>[2x]MDYKDDDDKWSHPQFEKHHHHHHHHWSHPQFEKQPPPPGPLGDCLRDWEDLQQDFQNIQETHRLYRLKLEELTKLQNNCTSSITRQKKRLQELALALKKCKPSLPAEAEGAAQELENQMKERQGLFFDMEAYLPKKNGLYLSLVLGNVNVTLLSKQAKFAYKDEYEKFKLYLTIILILISFTCRFLLNSRVTDAAFNFLLVWYYCTLTIRESILINNGSRIKGWWVFHHYVSTFLSGVMLTWPDGLMYQKFRNQFLSFSMYQSFVQFLQYYYQSGCLYRLRALGERHTMDLTVEGFQSWMWRGLTFLLPFLFFGHFWQLFNALTLFNLAQDPQCKEWQVLMCGFPFLLLFLGNFFTTLRVVHHKFHSQRHGSKKD

TMEM120A, a member of the transmembrane protein 120 (TMEM120) family, has a pivotal function in adipocyte differentiation and metabolism, and may also contribute to sensing mechanical pain by functioning as an ion channel named TACAN. HsTMEM120A forms a symmetrical homodimer with each monomer containing an amino-terminal coiled-coil motif followed by a transmembrane domain with six membrane-spanning helices. Each monomer contains an N-terminal soluble domain (NTD) on the cytosolic side and a transmembrane domain (TMD) embedded in a lipid bilayer. The TMD contains a bundle of six transmembrane helices (TM1-6) forming an asymmetric funnel with a wide opening on the intracellular side and a bottleneck on the extracellular side.

The cryo-EM structure of HsTMEM120A protein reconstituted in lipid nanodiscs forms a homodimeric assembly with an overall shape resembling a seesaw rocker. Unexpectedly, the HsTMEM120A protein reconstituted in nanodiscs contains a CoASH molecule per monomer that is from an endogenous cellular source and copurified along with the protein. Firstly, a small-molecule density is observed in the intracellular funnel-like cavity of each monomer and the density matches well with the CoASH model but not with the CoA derivatives (such as acetyl-CoA or fatty acyl CoA) or other nucleotide analogs. The CoASH molecule assumes a bent conformation and forms numerous specific interactions with amino acid residues on the lumen surface of the cavity. The 5-pyrophosphate and 3-phosphate groups of CoASH are positioned at the entrance of the cavity, while the adenosine and cysteamine groups of CoASH are inserted deep in the intracellular cavity pocket of HsTMEM120A in a key-lock mode. Trp193 of HsTMEM120A forms a strong π-π stacking interaction with the adenine group of CoASH. The blue dotted lines indicate the hydrogen bonds or the salt bridge between Lys130 NZ and CoASH O2B (3.6 Å), Lys130 NZ and CoASH O8A (3.4 Å), and Gln237 NE2 and CoASH N1A (3.8 Å). Mutation of the Trp193 to Ala dramatically reduced the affinity between CoASH and the protein. In the presence of CoASH, the intracellular cavity of HsTMEM120A is not only constricted by the four residues at the extracellular side but also blocked by the bulky adenosine 3-phosphate 5-pyrophosphate group of CoASH as well as its cysteamine and pantothenate groups. In case that TMEM120A does function as a mechanosensitive channel, the CoASH molecule may serve as a plug to block the intracellular entry and consequently stabilize the channel in a closed state, while the intracellular cavity may become accessible to ions upon dissociation of CoASH molecule from the cavity.> MRGSHHHHHHGRS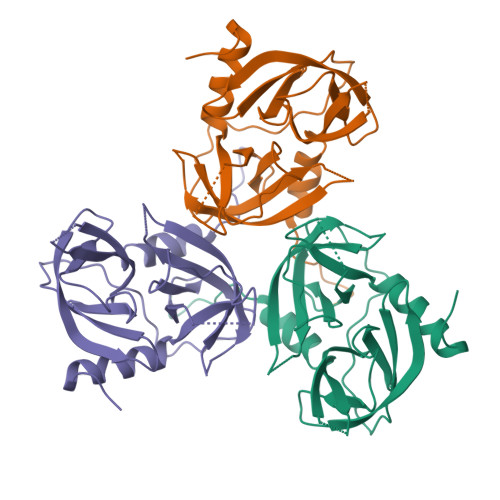LNPLSTPQFDSTDETPASYNLAVRRAAPAVVNVYNRGLNTNSHNQLEIRTLGSGVIMDQRGYIITNKHVINDADQIIVALQDGRVFEALLVGSDSLTDLAVLKINATGGLPTIPINARRVPHIGDVVLAIGNPYNLGQVITQGIISATGRIGLNPTGRQNFLQTDASINPGNSGGALVNSLGELMGINTLSFDKSNDGETPEGIGFAIPFQLATKIMDKLIRDGRVIR> SPSQMEHAMETMMFTFHKFAGDKGYLTKEDLRVLMEKEFPGFLENQKDPLAVDKIMKDLDQCRD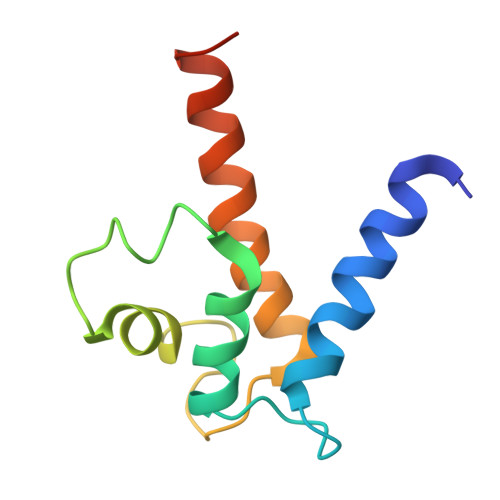GKVGFQSFFSLIAGLTIACNDYFVVHMKQKGKK>[4x]MNPAAEAEFNILLATDSYKVTHYKQYPPNTSKVYSYFECREKKTENSKLRKVKYEETVFYGLQYILNKYLKGKVVTKEKIQEAKDVYKEHFQDDVFNEKGWNYILEKYDGHLPIEIKAVPEGFVIPRGNVLFTVENTDPECYWLTNWIETILVQSWYPITVATNSR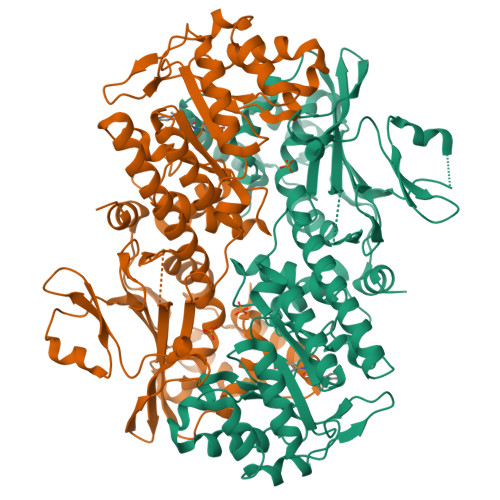EQKKILAKYLLETSGNLDGLEYKLHDFGYRGVSSQETAGIGASAHLVNFKGTDTVAGLALIKKYYGTKDPVPGYSVPAAEHSTITAWGKDHEKDAFEHIVTQFSSVPVSVVSDSYDIYNACEKIWGEDLRHLIVSRSTQAPLIIRPDSGNPLDTVLKVLEILGKKFPVTENSKGYKLLPPYLRVIQGDGVDINTLQEIVEGMKQKMWSIENIAFGSGGGLLQKLTRDLLNCSFKCSYVVTNGLGINVFKDPVADPNKRSKKGRLSLHRTPAGNFVTLEEGKGDLEEYGQDLLHTVFKNGKVTKSYSFDEIRKNAQLNIELEAAHHHHHHHH> SNAMDISVIDATKVNTETGLHIGESNAPVKMIEFINVRCPYCRKWFEESEELLAQSVKSGKVERIIKLFDKEKESLQRGNVMHHYIDYSAPEQALSA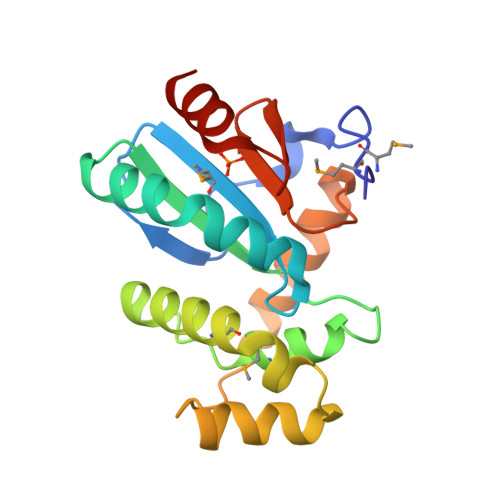LHKMFATQDEWGNLTLEEVATYAEKNLGLKEQKDATLVSAVIAEANAAHIQFVPTIIIGEYIFDESVTEEELRGYIEK>[10x]PGSIPLIGERFPEMEVTTDHGVIKLPDHYVSQGKWFVLFSHPADFTPVSTTEFVSFARRYEDFQRLGVDLIGLSVDSVFSHIKWKEWIERHIGVRIPFPIIADPQGTVAR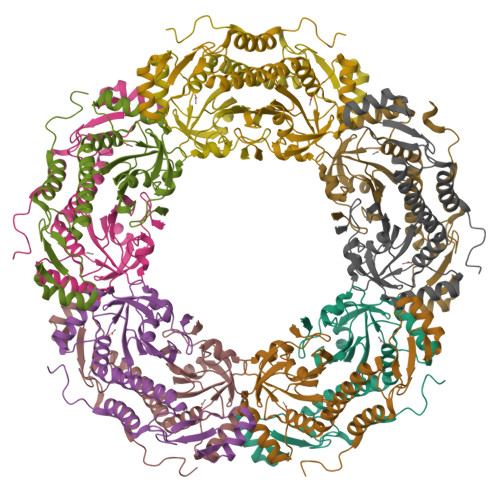RLGLLHAESATHTVRGVFIVDARGVIRTMLYYPMELGRLVDEILRIVKALKLGDSLKRAVPADWPNNEIIGEGLIVPPPTTEDQARARMESGQYRCLDWWFCWDTPASRDDVEEARRYLRRAAEKPAKLLYEEARTHLH>MSSSPCDQLQSFADGDLPPMEAQAFGQHLADCEKCQVELTRLLQLDQLGRGYIERHGPVDIPWHALPRNRWMAGGFALASMVAVAFILLGTLRPQAPRALPELWAQPQRTLEARVTYLAADRYRRPPQVMMGGAAARSGPNRSLALLSELEKRGDLHQLAVAYLATGVPEPSSAKAILEGMRSDLRWQSADVLCDLGVAHYVASKPLDAARATEELREALRLFDTVLAMQPGHVQALWNRSLVYRDLGLPLSAMKDLTEFEHRETDEGWRSEARDRRARLSSTLRRKERWLAADQTGADLINRGAQELARALTFVDVPLLRRDFYHAVRARTSSTDVLALLPLAERLDASVGSGTVLADYVHQVAARDFSRRAPLAEQYARLISGRIPESEQDALLQRFLTSDETDLALGALAHVMQRLPAYASELVRRTQHDEDPWFRVLGLQAQAMLERQQEHYKEALAPLEQALDICRRERLVYRCIFIENDLSHVKSWLFRVNAAAQHARDGLALARPNQWDLEGVMLQALGNVARQAADVTLGRAYYGEALLMAEGDKWSTRNIHQNLAHLAIWALELDEARASLDRAMDTGLPLTQHGVAALVDVARTRRSPRDALMVEQALAREPGNTPGQRAYAKFLHGRILVEVDPARGRMLLDEAIRQAEALPLDDVSAAHARAYSYTSLIFADADTGDFIAALARFGAELGFETPARCVLGLTADTERSLLVARGAQGQLLSAYVPLRSSRFEAASMEGAVPPEMLAALQACTLVDVLAR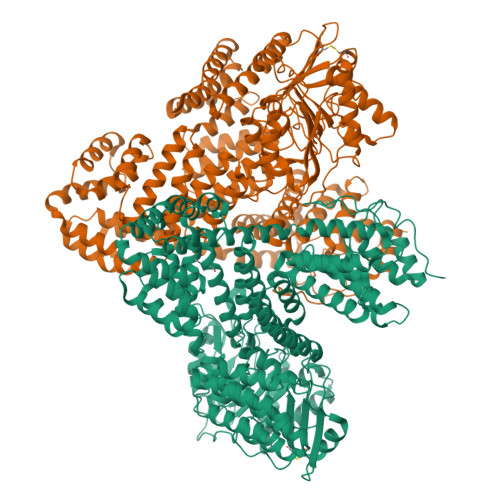PPLQGRSGLLPPGIAWRYRTRAAAPPPPAGPGTHLVVNEVRYSEERNEVPLQWLPRTAPGAEARFLRDLAATPTQVLEAISTATEIDLATHGKVDPDSNFAYLLLAPGADGRDTLFEDSIRASQLTGAPLVVLAACEGGRPNAALHRAGSLPSAFLAAGARAVLAATHPIPDLDSSAFFGAVRDRVLAGASLAVAVRDERLQWLSAGGDSEWVNAVLVFE[2x]>TPLVHVASVEKGRSYEDFQKVYNAIALKLREDDEYDNYIGYGPVLVRLAWHTSGTWDKHDNTGGSYGGTYRFKKEFNDPSNAGLQNGFKFLEPIHKEFPWISSGDLFSLGGVTAVQEMQGPKIPWRCGRVDTPEDTTPDNGRLPDADKDADYVRTFFQRLNMNDREVVALMGAHALGKTHL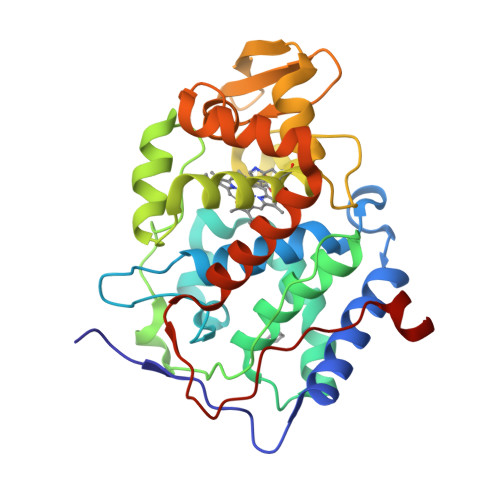KNSGYEGPWGAANNVFTNEFYLNLLNEDWKLEKNDANNEQWDSKSGYMMLPTDYSLIQDPKYLSIVKEYANDQDKFFKDFSKAFEKLLENGITFPKDAPSPFIFKTLEEQGL[4x]>EGAALTEKTDIFESGRNGKPNKDGIKSYRIPALLKTDKGTLIAGADERRLHSSDWGDIGMVIRRSEDNGKTWGDRVTITNLRDNPKASDPSIGSPVNIDMVLVQDPETKRIFSIYDMFPEGKGIFGMSSQKEEAYKKIDGKTYQILYREGEKGAYTIRENGTVYTPDGKATDYRVVVDPVKPAYSDKGDLYKGNQLLGNIYFTTNKTSPFRIAKDSYLWMSYSDDDGKTWSAPQDITPMVKADWMKFLGVGPGTGIVLRNGPHKGRILIPVYTTNNVSHLNGSQSSRIIYSDDHGKTWHAGEAVNDNRQVDGQKIHSSTMNNRRAQNTESTVVQLNNGDVKLFMRGLTGDLQVATSKDGGVTWEKDIKRYPQVKDVYVQMSAIHTMHEGKEYIILSNAGGPKRENGMVHLARVEENGELTWLKHNPIQKGEFAYNSLQELGNGEYGILYEHTEKGQNAYTLSFRKFNWDFLSKDLISPTEAKVKRTREMGKGVIGLEFDSEVLV[2x]

Streptococcus pneumoniae genomes encode three sialidases, NanA, NanB and NanC, which are key virulence factors that remove sialic acids from various glycoconjugates. Sialidases are one key virulence factor as they remove sialic acid from host cell-surface glycans, probably unmasking certain receptors to facilitate bacterial adherence and colonization. The 115 kDa NanA is the largest of the three sialidases and is anchored to the bacterial membrane. Although recombinantly expressed full-length NanA was soluble, it failed to crystallize; therefore, a 56.5 kDa domain that retained full enzyme activity was subcloned.

In this paper, we report the 2.5 Å resolution X-ray crystallographic structure of the catalytic domain of S. pneumoniae NanA and its complex with the inhibitor 2-deoxy-2,3-dehydro-N-acetyl neuraminic acid (Neu5Ac2en). Data were collected at 100 K to 2.5 Å resolution from a crystal grown in the presence of the inhibitor 2-deoxy-2,3-dehydro-N-acetyl neuraminic acid. The crystal belongs to space group P212121, with unit-cell parameters a = 49.2, b = 95.6, c = 226.6 Å. The two monomers in the asymmetric unit are related by a noncrystallographic twofold axis, superimpose with an r.m.s.d. of 0.39 Å over 470 Cα atoms and bury ∼1200 Å2 of surface at their dimer interface. The active site contains the usual catalytic residues common to all sialidases: three arginines (Arg347, Arg663, Arg721) that interact with the carboxylate group of sialic acid, a nucleophilic tyrosine (Tyr752) that is proposed to form a covalent intermediate and its associated glutamic acid (Glu647), an aspartic acid (Asp372) that acts as an acid/base and a hydrophobic pocket that accommodates the acetamidomethyl group of sialic acid. In common with other bacterial sialidases, the hydroxyl group at C4 on Neu5Ac2en interacts with an arginine (Arg366) and an aspartic acid (Asp417). The O8 and O9 hydroxyls of the ligand’s glycerol group interact with Tyr590 and Gln602, respectively. The topology of the surface of CNanA around the location of the aglycon is flat and open, in line with the promiscuity shown by NanA towards α(2,3), α(2,6) and α(2,8) linkages (unpublished data) and in contrast to leech sialidase and Trypanosoma cruzi trans-sialidase, which show specificity for α(2,3)-linked sialic acids. Two inhibitors of the influenza virus neuramini­dase, zanamivir and oseltamivir, are currently licensed as treatments for influenza and both were developed based on the framework of Neu5Ac2en. The study reported here lays the groundwork for the potential elaboration of the core of Neu5Ac2en, particularly around the acetamido and glycerol moieties, in order to develop specific inhibitors of the pneumococcal sialidases.> MAKNNAVAGFNALNGVELNLFTTDELKAIHYATMEVLMDPGIQVSDPEARQIFKENGCEVNEKTNVVKIPEYLVRKALQLAPSRFVLWGRDKKFN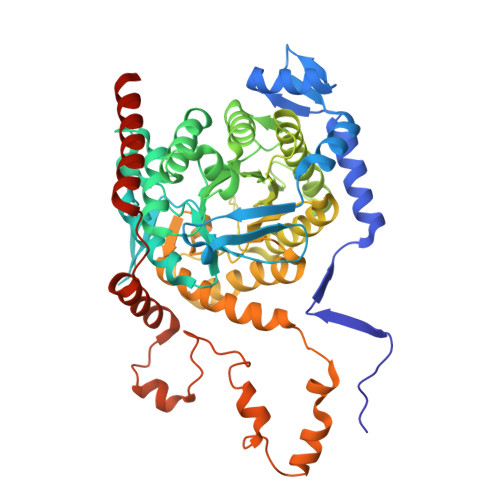TVQECGGKVHWTCFGTGVKVCKYQDGKYVTVDSVEKDIADIAKLCDWAENIDYFSLPVSARDIAGQGAQDVHETLTPLANTAKHFHHIDPVGENVEYYRDIVKAYYGGDEEEARKKPIFSMLLCPTSPLELSVNACQVIIKGARFGIPVNVLSMAMSGGSSPVYLAGTLVTHNAEVLSGIVLAQLTVPGAKVWYGSSTTTFDLKKGTAPVGSPELGLISAAVAKLAQFYGLPSYVAGSOSDAKVPDDQAGHEKTMTTLLPALAGANTIYGAGMLELGMTFSMEQLVIDNDIFSMVKKAMQGIPVSEETLAVESIQKVGIGNNFLALKQTRQLVDYPSNPMLLDRHMFGDWAAAGSKDLATVAHEKVEDVLKNHQVTPIDADIFKDMQAIVDKADKAFRGMGGHHHHHH>[2x]MRGSHHHHHHGSRSKFYES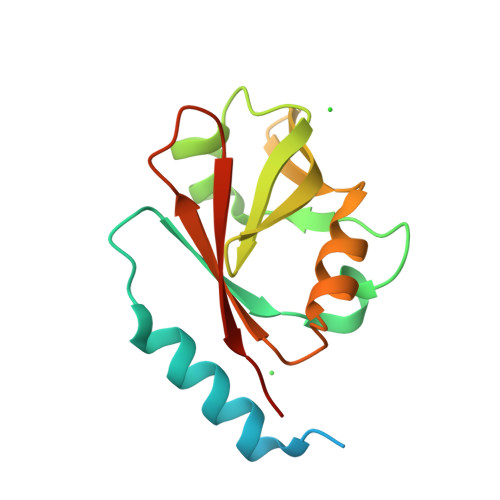ASARKRTVTAEERERAINAAKTFEPTNPFFRVVLRPSYLYRGCIMYLPSGFAEKYLSGISGFIKVQLAEKQWPVRCLYKAGRAKFSQGWYEFTLENNLGEGDVCVFELLRTRDFVLKVTAFRVNEYV> MKTMRKQIYKKAYWLLLPFLPLALANTFLVKEDSKNVTAYTPFATPITDSKSDLVSLAQLDSSYQIADQTIHNTNLFVLFKSRDVKVKYESSGSNNISFDSTSQGEKPSYVVEFTNSTNIGIKWTMVKKYQLDVPNVSSDMNQVLKNLILEQPLTKYTLNSSLAKEKGKTQREVHLGSGQANQWTSQRNQHDLNNNPSPNASTGFKLTTGNAYRKLSESWPIYEPIDGTKQGKGKDSSGWSSTEENEAKNDAPSVSGGGSSSGTFNKYLNTKQALESIGILFDDQTPRNVITQLYYASTSKLAVTNNHIVVMGNSFLPSMWYWVVERSAQENASNKPTWFANTNLDWGEDKQKQFVENQLGYKETTSTNSHNFHSKSFTQPAYLISGIDSVNDQIIFSGFKAGSVGYDSSSSSSSSSSSSTKDQALAWSTTTSLDSKTGYKDLVTNDTGLNGPINGSFSIQDTFSFVVPYSGNHTNNGTTGPIKTAYPVKKDQKSTVKINSLINATPLNSYGDEGIGVFDALGLNYNFKSNQERLPSRTDQIFVYGIVSPNELRSAKSSADSTGSDTKVNWSNTQSRYLPVPYNYSEGIIDADGFKRPENRGASVTTFSGLKSIAPDGFANSIANFSVGLKAGIDPNPVMSGKKANYGAVVLTRGGVVRLNFNPGNDSLLSTTDNNIAPISFSFTPFTAAESAVDLTTFKEVTYNQESGLWSYIFDSSLKPSHDGKQTPVTDNMGFSVITVSRTGIELNQDQATTTLDVAPSALAVQSGIQSTTQTLTGVLPLSEEFSAVIAKDSDQNKIDIYKNNNGLFEIDTQLSNSVATNNGGLAPSYTENRVDAWGKVEFADNSVLQARNLVDKTVDEIINTPEILNSFFRFTPAFEDQKATLVATKQSDTSLSVSPRIQFLDGNFYDLNSTIAGVPLNIGFPSRVFAGFAALPAWVIPVSVGSSVGILFILLVLGLGIGIPMYRVRKLQDASFVNVFKKVDTLTTAVGSVYKKIITQTGVVKKAPSALKAANPSVKKPAAFLKPPVQPPSKPEGEQKAVEVKSEETKS;> MHQPKKRLAKKSWAFLTAALTLGVITGVGGYFLFNQNKQRSSVSNFAYQPKQLSVKHQQAVDETLTPWTWNNNNFSSLKITGENPGSFGLVRSQNDNLNISSVTKNSSDDNLKYLNAVEKYLDGQQNFAIRRYDNNGRALYDINLAKMENPSTVQRGLNGEPIFDPFKGFGLTGNAPTDWNEIKGKVPVEVVQSPHSPNLYFVLLVPKVALEYHNLNNQVVKESLEVKATQSSFNPTQRLQKDSPVKDSSKQGEKLSETTASSMSSGMATSTRAKALKVEVERGSQSDSLLKNDFAKKPLKHKNSSGEVKLEAEKEFTEAWKPLLTTDQIAREKGMGATVVSFYDAPYSENHTAFGLVDHIDPKKMVENYPPSWKTPKWNHHGIWDYNARNLLLQTTGFFNPRRHPEWFDEGQAKADNTSPGFKVGDTDHKKDGFKKNSSSPIALPFEAYFANIGNMVAIGNSVFIFGGNGHATKMFTTNPLSIGVFRIKYTDNFSKSSVTGWPYAVLFGGLINPQTNGLKDLPLGTNRWFEYVPRMAVSGVKWVGNQLVLAGTLTMGDTATVPRLKYDQLEKHLNLVAQGQGLLREDLQIFTPYGWANRPDIPVGAWLQDEMGSKFGPHYFLNNPDIQDNVNNDTVEALISSYKNTDKLKHVYPYRYSGLYAWQLFNWSNKLTNTPLSANFVNENSYAPNSLFAAILNEDLLTGLSDKIFYGKENEFAENEADRFNQLLSLNPNPNTNWARYLNVVQRFTTGPNLDSSTFDQFLDFLPWIGNGKPFSNSPSPSTSASSSTPLPTFSNINVGVKSMITQHLNKENTRWVFIPNFSPDIWTGAGYRVQSANQKNGIPFEQVKPSNNSTPFDPNSDDNKVTPSGGSSKPTTYPALPNSISPTSDWINALTFTNKNNPQRNQLLLRSLLGTIPVLINKSGDSNDQFNKDSEQKWDKTETNEGNLPGFGEVNGLYNAALLHTYGFFGTNTNSTDPKIGFKADSSSSSSSTLVGSGLNWTSQDVGNLVVINDTSFGFQLGGWFITFTDFIRPRTGYLGITLSSLQDQTIIWADQPWTSFKGSYLDSDGTPKSLWDPTALKSLPNSSTTYDTNPTLSPSFQLYQPNKVKAYQTTNTYNKLIEPVDATSAATNMTSLLKLLTTKNIKAKLGKGTASSQGNNNGGGVSQTINTITTTGNISEGLKEETSIQAETLKKFFDSKQNNKSEIGIGDSTFTKMDGKLTGVVSTPLVNLINGQGATSDSDTEKISFKPGNQIDFNRLFTLPVTELFDPNTMFVYDQYVPLLVNLPSGFDQASIRLKVISYSVENQTLGVRLEFKDPQTQQFIPVLNASSTGPQTVFQPFNQWADYVLPLIVTVPIVVIILSVTLGLTIGIPMHRNKKALQAGFDLSNKKVDVLTKAVGSVFKEIINRTGISNAPKKLKQATPTKPTPKTPPKPPVKQ

The nap particle is an immunogenic surface adhesion complex from Mycoplasma genitalium. It is essential for motility and responsible for binding sialylated oligosaccharides on the surface of the host cell. Cryo-electron tomography (cryo-ET) of M. genitalium revealed the tetrameric organization of the nap particle complex, consisting of two P140-P110 heterodimers. The P140-P110 heterodimers form the ‘tight interface’, while the ‘loose interface’ is formed between the two heterodimers.

In contrast to previous studies, this analysis by classification of the native nap particle displayed both the ‘open’ and the ‘closed’ state of the tight interface, resolved at 17 Å and 18 Å, respectively. (c) Top view of the surface representation of the closed conformation of the P140 (blue)-P110 (yellow) heterodimer. (d) Enlarged view of the binding pocket illustrates hydrogen bonds formed between the P110 and P140. In this state, binding of 6′-SL is not possible. In the ‘closed’ conformation, there is no density seen at the loose interface, whereas in the ‘open’ conformation, P110 and P140 come into proximity at the loose interface, thus indicating an interaction between loop 662–666 of P110 and loop 1173–1179 of P140. In fact, classes showing an opening and closing of the tight interface are always associated with a repositioning of the P110 stalk. Intracellular signaling, likely at the intracellular region of P140, then triggers a conformational change within the P140 stalks, changing the angle of the heterodimers relative to each other and thus transitioning to the expanded conformation where P140 and P110 do not interact at the loose interface. This allows P110 to reposition the stalk and close the tight interface, resulting in the "closed" conformation where no sialylated oligosaccharides can be bound. Despite classification efforts, the intracellular region does not display differences between the ‘open’ and ‘closed’ state.>GPMPGLSVKLRVAEAYPEDVGKGIVRMDKASRAKLGVSVGDYVEVKKVLSVKLRVAEAYPEDVGK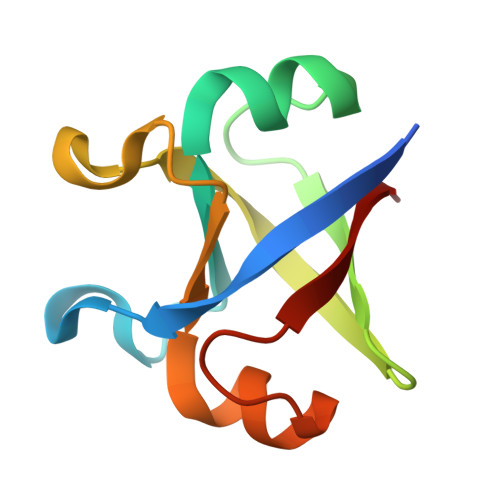GIVRMDKASRAKLGVSVGDYVEVKKV[2x]> HHHHHHGSARDISSTNVTDLTVSPSKIEDGGKTTVKMTFDDKNGKIQNGDMIKVAWPTSGTVKIEGYSKTVPLTVKGEQVGQAVITPDGATITFNDKVEKLSDVSGFAEFEVQGRNLTQTNTSDDKVATITSGNKSTNVTVHKSEAGTSSVFYYKTGDMLPEDTTHVRWFLNINNEKSYVSKDITIKDQIQGGQQLDLSTLNINVTGTHSNYYSGQSAITDFEKAFPGSKITVDNTKNTIDVTIPQGYGSYNSFSINYKTKITNEQQKEFVNNSQAWYQEHGKEEVNGKSFNHT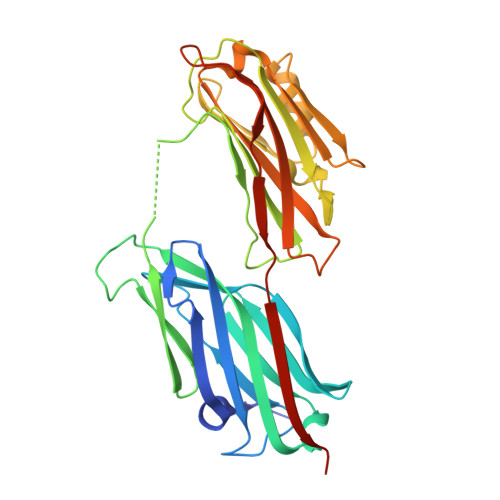VHNINANAGIEGTVKGELK>GSHMGVQHKLDIFLVSEGIAIKEANLLKGDSYGCTIKIKLDKEKTFKFVIVLEPEWIDEIKPIYMKVNDESVELELDYKDATKRIYSAEVVLSSDSVINLFSDVDVSYTSEYPTIKVNTIKKYYSVQNRGMTYVHIESPINTKDKSWFVEKNGWYEDRT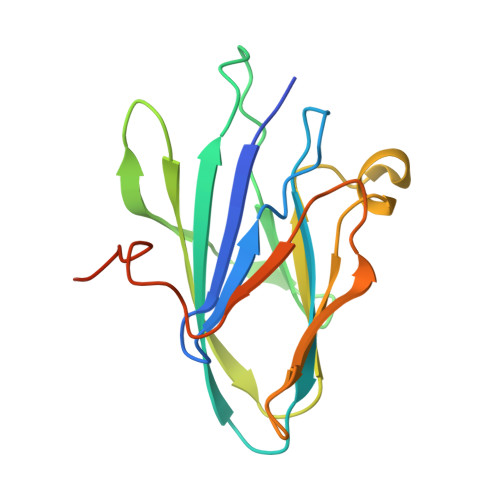HS[2x]>[5x]YKDDDDKLHSQANLMRLKSDLFNRSPMYP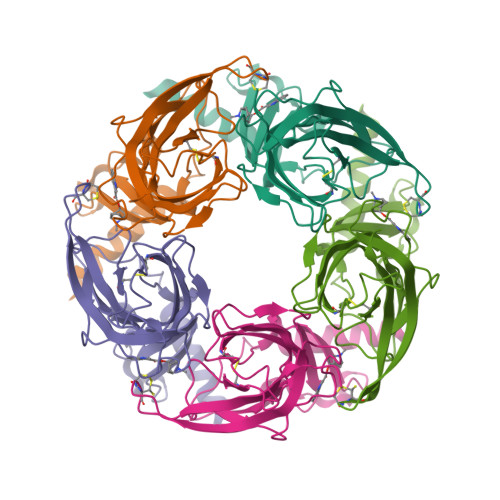GPTKDDPLTVTLGFTLQDIVKADSSTNEVDLVYYEQQRWKLNSLMWDPNEYGNITDFRTSAADIWTPDITAYSSTRPVQVLSPQIAVVTHDGSVMFIPAQRLSFMCDPTGVDSEEGATCAVKFGSWVYSGFEIDLKTDTDQVDLSSYYASSKYEILSATQTRQVQHYSCCPEPYIDVNLVVKFRERRAGNGFFRNLFD> MDVPADSHIKYEDAIDYWTDVDATVDGVLGGYGEGTVVPTMDVLGSNNFLRKLKSRMLPQENNVKYAVDIGAGIGRVSKTMLHKHAAKIDLVEPVKPFIEQMHVELAELKDKGQIGQIYEVGMQDWTPDAGKYWLIWCQWCVGHLPDAELVAFLKRCIVGLQPNGTIVVKENNTPTDTDDFDETDSSVTRSDAKFRQI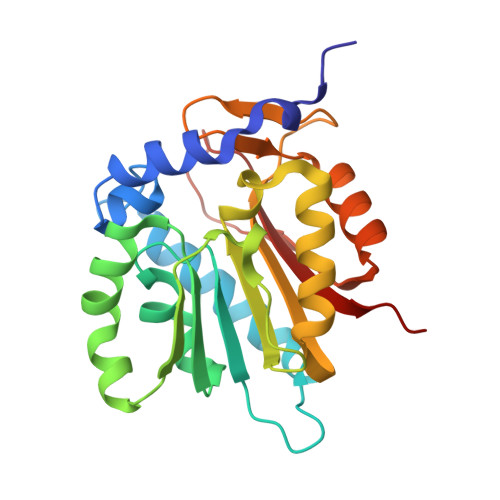FEEAGLKLIASERQRGLPRELYPVRMYALKPMPN>[2x]AMITEKSAALYARAVEVMPGGNSRTAVYSSPYPVYVRSGSGARVTDVDGVERIDFLNNSTTLIHGHAHPEMVEAIAAAVGHGTSFGMPTPVEVEYAEALSARNETFEHVRFTSSGTEAVMMAVQAARAYTERPKIAKIAGAYHGAYDAVAVNNDGSGNLISHAVTGNPEGVVANTVVIPFNDPEGSLEVLRRHADDLACVLIDPVPWRIGLLPASKEWLDALREFCDASGAVLISDEVGSYRVGYHGAMQLLGAEADITVMGKVIAAGMPIGAVAGRRRFMSVFDPSKGKPALPHSGSYNANPVSMSSGIASLRLLTPQAHERIGQLGEQARGSMRTALGEAGLDWEVNGLGSLFRVVANSAPAGYDSAAAAMKALYWKLLENGIHIGDSGLGCISTPMGEEEIAEYAVAFAKSLGQVLAEGRA

As part of investigations into the C-nucleoside formycin A (8-aza-9-deazaadenosine) biosynthetic gene cluster from Streptomyces kaniharaensis, we have characterised a pyridoxal 5′-phosphate (PLP) dependent aminotransferase (ForI) that aminates a pathway intermediate. ForI is a PLP-dependent enzyme from the biosynthetic pathway of the C-nucleoside antibiotic formycin. ForI possesses the mixed β-sheet and three-stranded antiparallel β-sheet insertion characteristic of the PLP dependent aspartic aminotransferase family. The predicted active site of ForI comprises residues from two monomers, indicating the dimer to be the functional unit.

Incubating ForI with l-Glu shows a rapid change in the UV-vis spectrum (ESI†). We incubated crystals of ForI with l-Glu for 20 minutes and collected a 1.56 Å resolution data set. The electron density clearly indicates that the pyridoxal co-factor is unattached to the enzyme, suggesting it to be PMP. Despite numerous attempts we have not observed density for l-Glu or α-KG. PMP forms a 3.2 Å hydrogen bonding interaction with ε-N of Lys 262. The plane of the PMP molecule has rotated by 22° relative to PLP. Residues Tyr 141 and Trp 206 are slightly displaced, Arg 207 switches to an alternate conformation. Accompanying these changes in protein structure are shifts in water molecule locations. These structural changes result in the pocket adjacent to the cofactor (bounded by Ala 25, Thr 60, Tyr 141, Trp 206) enlarging further and becoming more open to solvent.> MGLNFFRKAAPEVRTEPVAERKASVTGRI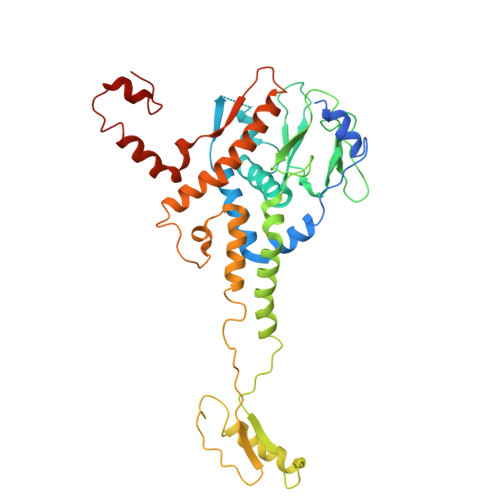VAMASGAGRPVWGPRDTVSLMRTGFAGNPVGFRSVKLIAEATAAVPLICQDAERRYEIHPVLDLLRRPNAGQGRAELFEALIGQILLSGNGYLEAVCPEPGVPRELHVLRSDRMAVVPGADGWPVGYDYTVGGRKHRFDMTGHPDPICHIKSFHPTDDHYGLSPMQAAAVALDVHNAASAWSKALLDNAARPSGAIIYKGADGQGVLAPEQYERLIFEMETHHQGARNAGRPMLLEGGLDWKPMGFSPSDMEFHETKAAAAREIALAFGVPPMLIGIPGDATYANYAEANRAFYRLTVLPLLTRVSAALAWWLSGYLGAQIELKPDLDQVPALAVERDQLWARIGAAGFLSNSEKRVLLGLPPTAEG>[2x]MDWALFLTFLAACGAPATTGALLKPDEWYDNLNKPWWNPPRWVFPLAWTSLYFLMSLAAMRVAQLEGSGQALA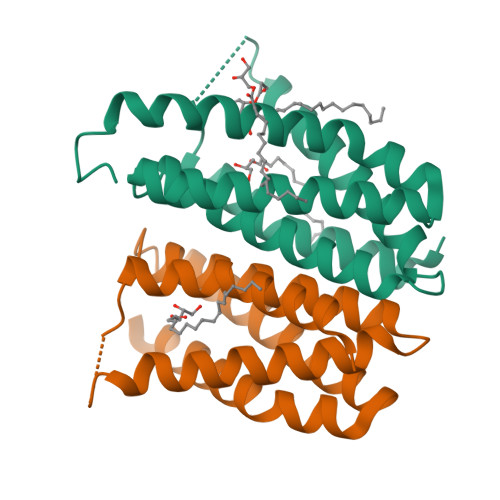FYAAQLAFNTLWTPVFFGMKRMATALAVVMVMWLFVAATMWAFFQLDTWAGVLFVPYLIWATAATGLNFEAMRLNWNRPEAR> SAIASNVRVLATDLAFPEGPVVMPDGSVVLVEIRAQQLTRVWPDGRKEVVAKVPGGPNGAALGPDGKMYICNNGGFGWFPSRGTMMPGAPAPHEYIGGSIQRVDLQSGEVETLFDKCGEHPLKGPNDLVFDKHGGLWFTDLGKRRARDMDVGAAYYIKPGMTEITEQVFGTLPLNGIGLSPDEATMYAAETPTGRLWAFDLSGPGEVKPRDVIYRGEKGKPICGLGGYQMFDSLAVEASGNVCVATLVSGCISVIAPDGTLVEQVPTGDRVTTNIAFGGPDLKTAYITLSGKGELIAMDW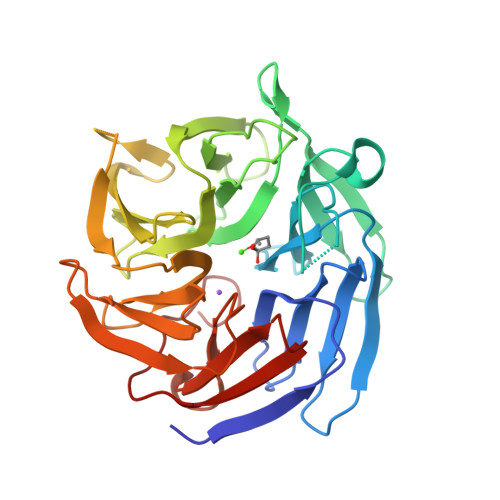SRPGLPLNFLNK>[2x]VSPKTYKDADFYVAPTQQDVNYDLVDDFGANGNDTSDDSNALQRAINAISRKPNGGTLLIPNGTYHFLGIQMKSNVHIRVESDVI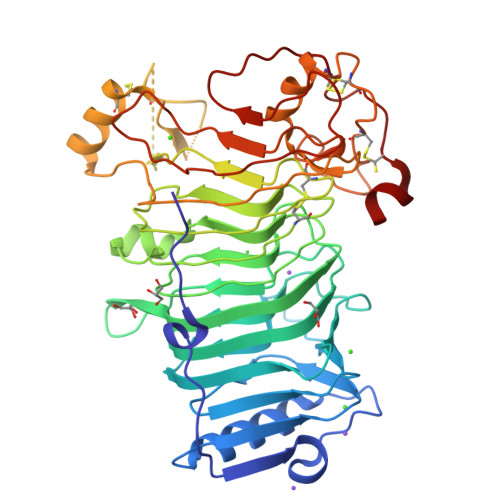IKPTWNGDGKNHRLFEVGVNNIVRNFSFQGLGNGFLVDFKDSRDKNLAVFKLGDVRNYKISNFTIDDNKTIFASILVDVTERNGRLHWSRNGIIERIKQNNALFGYGLIQTYGADNILFRNLHSEGGIALRMETDNLLMKNYKQGGIRNIFADNIRCSKGLAAVMFGPHFMKNGDVQVTNVSSVSCGSAVRSDSGFVELFSPTDEVHTRQSWKQAVESKLGRGCAQTPYARGNGGTRWAARVTQKDACLDKAKLEYGIEPGSFGTVKVFDVTARFGYNADLKQDQLDYFSTSNPMCKRVCLPTKEQWSKQGQIYIGPSLAAVIDTTPETSKYDYDVKTFNVKRINFPVNSHKTIDTNTESSRVCNYYGMSECSSSRWER> MGSSHHHHHHSSGLVPAGSHMSKLASSSVCDSTIENPCIVQDSKTQFSPVIRYREVASIADVYGGNITGINKFHLSGSEQPSEKGWEAIAESISRKMGPETKKVIVLDLRQESHGYLNGRAITLVSVYNWINLGKSNSQSTLDQENWLTGLRSRKIVNGVLTVPQYVAKQYSQGKSMVVSTVKNEEYYVYKKGFDYYRIFISDHRAPLDSEVDALVALIKNNPEDTWYHVHSRGGKGRTTTVFAMFDMLKNADKVSFEEIIARQASIPPFYNLMVTNREIPELTPYYEQRLQFLIHF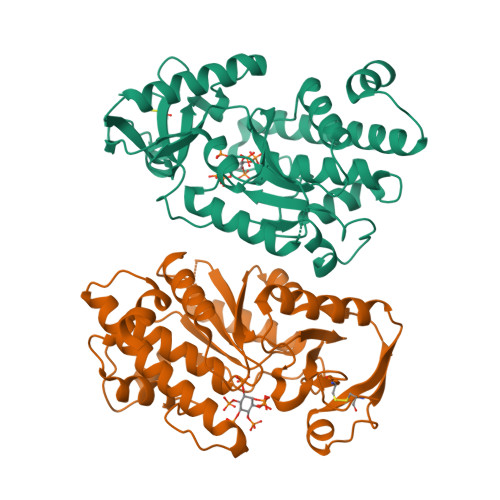YEFARQSLMGYSGTWSEWKKLNI>GFPSPAADYVEQRIDLNQLLIQHPSATYFVKASGDSMIDGGISDGDLLIVDSAITASHGDIVIAAVDGEFTVKKLQLRPTVQLIPMNSAYSPITISSEDTLDVFGVVIHVV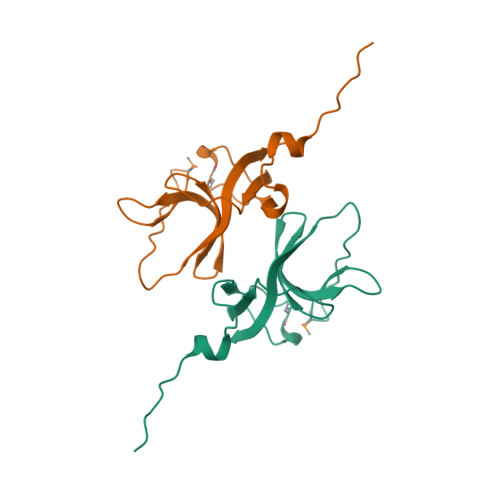KAATR[2x]>[2x]MSKKNVDPFSDSDSSSEPPSIFSSDNEENSDVDNSVIINDKNTKSDEADIKYMDEDESSDSESESESKKKSKKSKKSKKSKKSVTKKKNNLLVGNRIITEYILIDANNYHFKSWIECFPDCKVNLKLLLFRPEWFDFFKYVESKTYFPQLESKLSSYLEKRQRIVPYPELLFNTMNVLPPGKIKVVILGQDPYPGSCISGVPYAMGCSFSVPLNCPVPKSLANIYTNLIKFNHMRKAPKHGCLASWILQGTFMINSAFTTVLNESGVHARTWESFTADLIDYLTDNYDDLIFVAWGAHAHKLCQRVDPKKHYIITSSHPSPYSVSNTMTSMSYGPNPKKVTYPSFNSVDHFGKINEHLKSRNKKPIFWDL

In the BER pathway, uracil-DNA glycosylase (UDG) recognizes uracil which exists in DNA and creates an abasic site by cleaving the N-glycosidic bond between uracil and deoxyribose. Interestingly, APMV UNG (mvUNG) is longer than other known UNGs, suggesting that it contains domains or motifs in addition to the canonical catalytic domain. mvUNG (residues 1–370) contains a catalytic domain conserved among UNG family proteins. Additionally, it has an N-terminal domain (N-domain; residues 1–130) and an insertional motif (motif-I; residues 327–343).

Needle-shaped crystals were grown from full-length mvUNG, and the diffraction data were collected up to 2.3 Å resolution. Residues 95–370 of two mvUNG proteins in the asymmetric unit were traced into the electron density, and the final model was refined with R/Rfree values of 17.3/21.6%. Thus, the N-terminal residues seem to be truncated before crystallization. Two mvUNGs in the asymmetric unit were superimposed with a root-mean-square deviation (RMSD) of 0.4 Å for 276 Cα atoms, indicating that the two mvUNGs are in the same conformation. The catalytic domain of mvUNG also forms a similar fold, comprising a central β-sheet (S2, S3, S5) sandwiched by α-helices (H5–H12). In the structure of mvUNG, residues 95–130 comprise four short helices, two α-helices (H1 and H3), and two 310-helices (H2 and H4). Residue R96 in the N-domain forms an ionic interaction with E169 in the catalytic domain, and the segment is fitted into a hydrophobic groove of the catalytic domain. Residues 95–130 of the N-domain seem to stabilize the catalytic core domain by binding to its hydrophobic surface. Motif-I forms a two-stranded antiparallel β-sheet (S7 and S8) and provides a positively charged surface near the active site, which might improve the interaction with the DNA backbone. The catalytic residue (D191) and the other four residues for uracil-binding specificity in the binding pocket (Y193, F209, N255, and H318) are conserved as the canonical active site residues, whereas Leu in the minor groove intercalation loop is replaced by Y322 in mvUNG.> ETGEVTLLDSRSVQGELGWIASPLEGGWEEVSIMDEKNTPIRTYQVCNVMEPSQNNWLRTDWITREGAQRVYIEIKFTLRDCNSLPGVMGTCKETFNLYYYESDNDKERF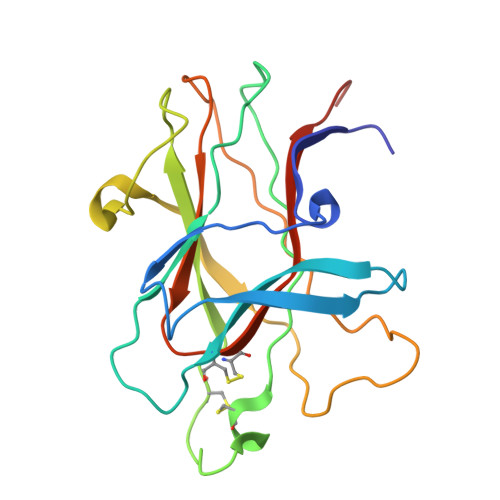IRENQFVKIDTIAADESFTQVDIGDRIMKLNTEIRDVGPLSKKGFYLAFQDVGACIALVSVRVFYKRTKHHHHHH> NPVENYIDEVLNEVLVVPNINSSNPTTSNSAPALDAAETGHTSSVQPEDVIETRYVQTSQTRDEMSLESFLGRSGCIHESKLEVTLANYNKENFTVWAINLQEMAQIRRKFELFTYTRFDSEITLVPCISALSQDIGHITMQYMYVPPGAPVPNSRDDYAWQSGTNASVFWQHGQAYPRFSLPFLSVASAYY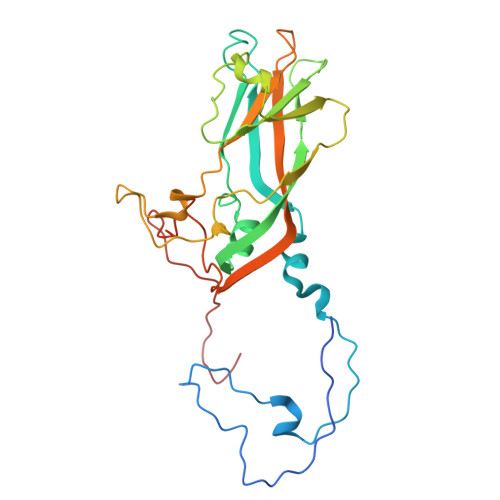MFYDGYDEQDQNYGTANTNNMGSLCSRIVTEKHIHKVHIMTRIYHKAKHVKAWCPRPPRALEYTRAHRTNFKIEDRSIQTAIVTRPIITTAGPSDMY>MEKPEFDPILLRPVDDLELTVRSANCLKAEAIHYIGDLVQRTEVELLKTPNLGKKSLTEIKDVLASRGLSLGMRLENWP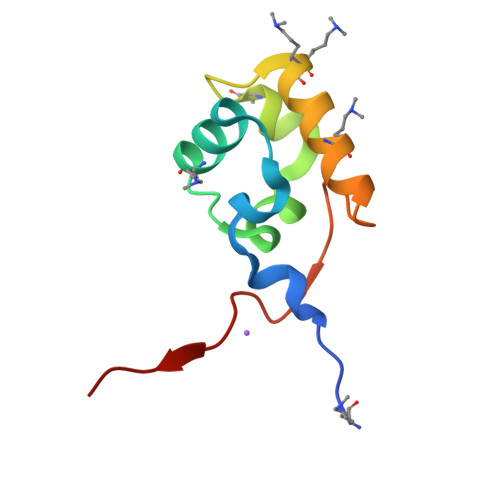PASIADE[8x]> MNTNSNTMVMNDANQAQITATFTKKILAHLDDPDSNKLAQFVQLFNPNNCRIIFNATPFAQATVFLQMWQNQVVQTQHALTGVDYHAIPGSGTLICNVNCKVRFDESGRDKMGQDATVPIQPNNTGNRNRPNDMNKPRPLWGPYFGIS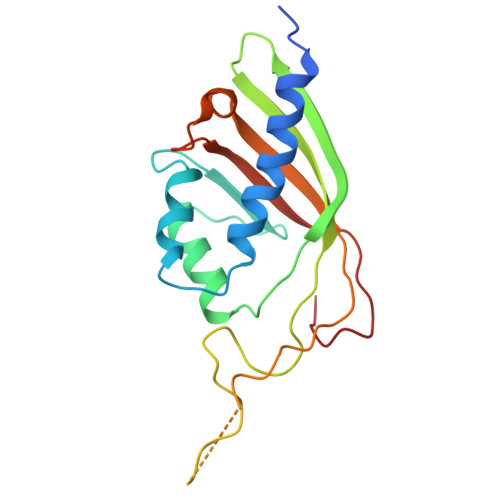LQLIIDDRIFRNDFNGVISGFNYNMVYKPEDSLLKI>GQGQETLTASRLASAPPQKQKQMLGERLFPLIQAMHPTLAGKITGMLLEIDNSELLYMLESPESLRSKVDEAVAVLQAHQAKEATQKAVN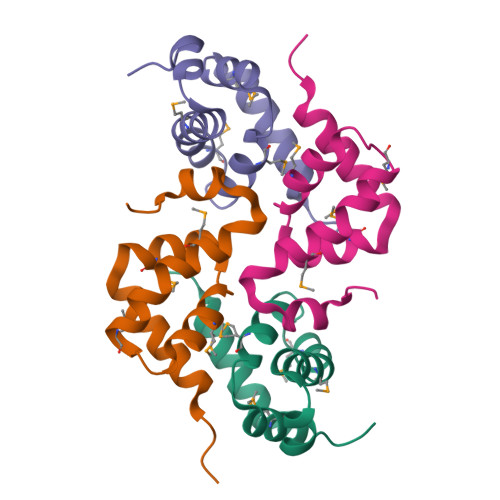SATGVPTV[4x]> GSHMANLDRTDDLVYLNVMELVRAVLELKNELSQLPPEGYVVVVKNVGLTLRKLIGSVDDLLPSLPSSSRTEIEGTQKLLNKDLAELINKMRLA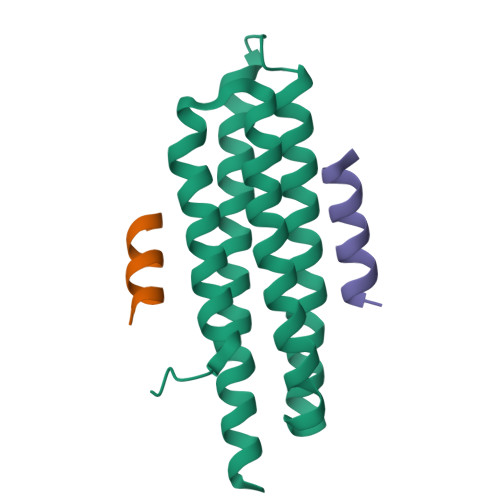QQNAVTSLSEEAKRQMLTASHTLAVDAKNLLDAVDQAKVLANLAH;>GSNLSELDRLLLELNAVQHNPPSG[2x]> MLKIISANVNGIRSAY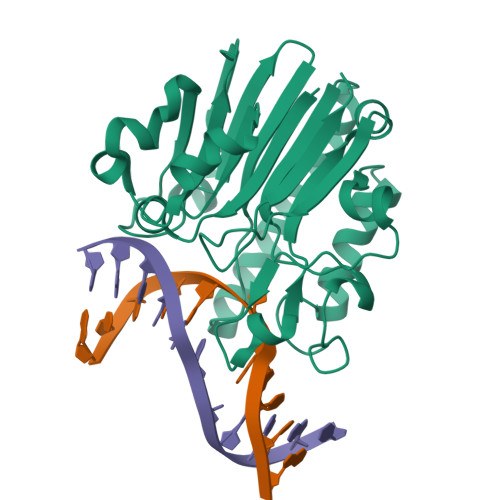KKGFYEYIAASGADIVCVQELKAQEADLSADMKNPHGMHGHWHCAEKRGYSGVAVYSKRKPDNVQIGMGIEEFDREGRFVRCDFGRLSVISLYLPSGSSAEERQQVKYRFLDAFYPMLEAMKNEGRDIVVCGDWNIAHQNIDLKNWKGNQKNSGFLPEEREWIGKVIHKLGWTDMWRTLYPDVPGYTWWSNRGQAYAKDVGWRIDYQMVTPELAAKAVSAHVYKDEKFSDHAPLVVEYDYAAE> KRNPDAGVATAVQSVIQHQTFKRMLLFGLRSLADFCSPSNQLYQENALDALDRGVLSAIQTAVTTFSDDDDLMLCASRVLWAMSVAIKEEMDPAHIARVHSEGSPVIVAVVNSSPTDPQTIEDSMNFVDNLKRAGAPVDGASLAGGMLSIFTKTALDMKTAKRVTAALAIAAETAEGSTALYNAGGTSVLLTYCLDQGDLSDAGVEMVEGAFDTVRYMAGYQCTDATTLPQCIALMDKYRGRKSASAKGSSALAAMIGPEQLQKCLNTLKTAEAGSAEYDEALVTLGSMSYISSFTDEIVRAGGVPLLIELINSGLPQMEGNPEKIASMISGAAKMLARIASNPVNVDAIVQAGGVATLCTAVSYCTESMEALGALCMALVPLASRESLAHEIVQYQTFATVLPILYQNVESPEIAALAMELVATGSQHEEIQEHMLQNQAAEICSLCCQYHTADASYQQHAISALNRLVPRLTTLHGVSEYGGIQGVIASLNANVNNEQVALLAVQLLDNFSEVSDAKTYMSDGTCVDAVLAAMLEHEGNDLLISAGVHCLARIATEDDCARHLNVLDTAIQTARGNPDGVYRVLAAISGLSRVPSLRQIFEEKNASDTILAGISSWIECSRFEGQNRIIKAALKTVKNMKISGDGDLTSCFAAMCDVACLPQVKRVVELEEPDNNILVADTAAFRDLAATMRITGAENLERCIESVLRVMRKYPDSRRAQLNCLETLNYLAQCDGGEGVAILSRTGGLNAVVQYLTRAPMYLDAQIAGFTVLATSAKIDSNVGETLRKCNCLQALKVAMRTHAKSKELKRTIAPLVALLMPTDALETEIQELLNECASACEKNNFPHLHENLAALNELLISSEGAKIAARLGIGAHMCKYQEYISAHEQDALAVTDYDILGKDLFDATVSECAHAMEQVASTRSGRNALIKAGNVATLISLYESLKAPQSQYSEEAAIHCLEALRILLKSDKRSAELAFERNFVSTLCVGIDSFPHSAPVLGATCACLAAMATTPERVQMLTAQPAFESLLQKLVFVIQNDPSKDNKLVAMRALQELVEITNDATMANKIAEAGAVTALFRIIDEYGDDEQLTVQAAEVLALLGAFEDLRRFYDNDVRFPAQVLTAALTKQKNNETAVVHLLDVLNKLATSEDRAVLRELGVMEQVADAMRVHSESEAVTRLGGELFAKMGADEQIKSLMLQIIETVESGAEDTAQTVDILCGRLAVFLAAPLEDPRDALQHTEKCLGSLVATLQTYPGSERLEGNVALVCRRLCDRCFDDADDPYGAWAVAASGMLAQFAGMVAGETVLANKKFLGPAYRTFTACCANAYCMPTMVEVAPSFLPQTYTLLEMHKNDAETVARVLEFLRYFAEDPTACGLIVQNMSGSSGDVVALTVLLMQQHQNNDAVVCAGMEFLGALAYTLSQAGYEPLPTLADGSVLRDCDALMGSNSSSARQLAHMHMIEKMLLSKAYNDALIQEQALKKLTMSLKAEDDKKRFSDEERAG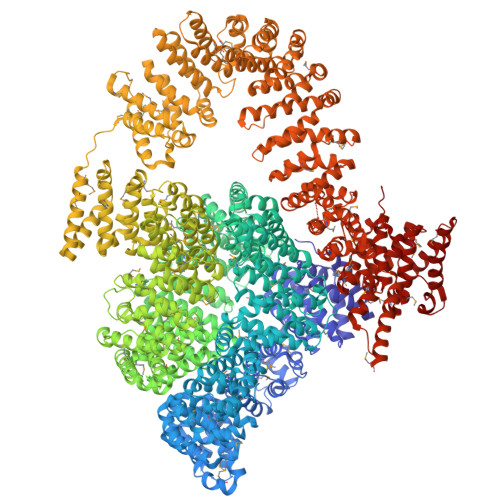LYAAMACVLLAAGGAGLTGEMEKFNGFEVVLQAIEEFGENPTVIKEVNRALQGLSMADVNMTARTVKEAVPKLCTEATTAIQTDAECADTFCDLMLQLVSQEGNGRQLLQVYGLEETLQGVENLAAYYGEDFGTQLSEKVAMIRQAMEDDQPREKTCKDVYDLLNSRVQQGLSVAISEVAILQEEVEFLVSQMGMYNQEQLDHQTAMGADHQYGNMAFELLAATSANVKLLQANEFSKMELALIKGQADPEIVLYAVKALTAFCKFPPAAQDTARIQGCPALVTEACSKINKSGLPNERKEEHLCARYFLVERTAINRNLYNKTPIMTELINSWNDYDKGAYTTTLLRFVFRAMRRVVSDAHVEELLKANVLQRLIGIISDVNADMALLPDVLFLLGSLAVVPEIKTKIGELNGIAACTDLLQRALPKPNTAPVVTNVCLAFANICIGHKKNTEIFSKLGGPALNVKVLNDRGHEYDVCNAASVLLCNLLYKNESMKKLLGTNGAPAALVKGLSNYDGSEEKTAIRCLESVFKAISNLSLYTPNIQPFLDAGIENAYSTWLSNLSETFPDAQLETGCRTLVNLVMENEENNMRKFGVCLLPCMAVAKQGRTDTKALLLLLDIEASLCRLKENAEAFAANGGIETTIRLIHQFDYDVGLLTLGIHLLGIQSAVKDSIQRMMDADVFSILVGCVEVDAEGNEVTDLVVGGLRCTRRIVRSEELAFEYCNAGGIATIANVICKSINQPMVMLEACRVLLGLLFYTTRSQADRQAAVEALHAQCQQRAEQMHAQAQADYEAGVVSEPPPEEMEVPEPDPDELANAAYGGWYQMGMDEVMIDAILQAVCACAAVEAHAKQLRLQRVCLGLAAYFASEQMGTSSLVGSGIEQVLTQIMTNFAGEGTTMQLSCVIINSIAMTSGDMYEEIKTSALLSALKTSVGKMATKKPEEKALKETCAATLEAASSGEDPFDAFSKTVTELDFKFTEWNVDPYP>[2x]GAMAPVASASPKLCLAWQGMLLLKNSNFPSNMHLLQGDLQVASSLLVEGSTGGKVAQLKITQRLRLD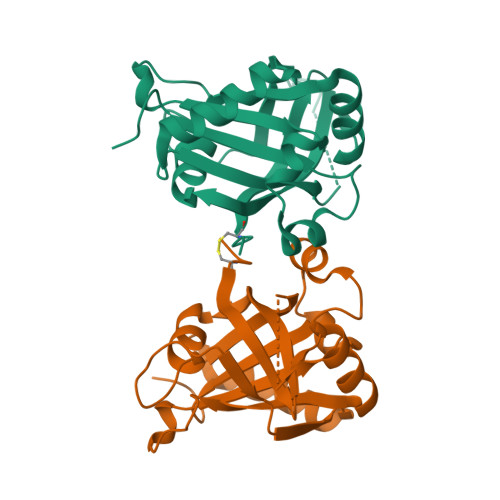QPKLDEVTRRIKVAGPNGYAILLAVPGSSDSRSSSSSAASDTATSTQRPLRNLVSYLKQKQAAGVISLPVGGNKDKENTGVLHAFPPCEFSQQFLDSPAKALAKSEEDYLVMIIVRGFGFQI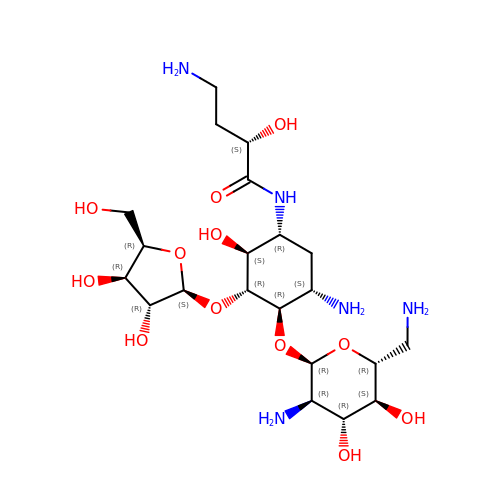(2S)-4-amino-N-[(1R,2S,3R,4R,5S)-5-amino-4-[(2,6-diamino-2,6-dideoxy-alpha-D-glucopyranosyl)oxy]-2-hydroxy-3-(beta-D-xylofuranosyloxy)cyclohexyl]-2-hydroxybutanamide | C21 H41 N5 O12 | XEQLFNPSYWZPOW-SVRMBHBBSA-N>[2x]XETAAFAALRKPVDVAFGRNYVPTWAFDHIKYFNGGNEIQLHLDKYTGTGFQSKGSYLFGHFSMQMKLVPGDSAGTVTAFYLSSQNSEHDEIDFEFLGNRTGQPYIL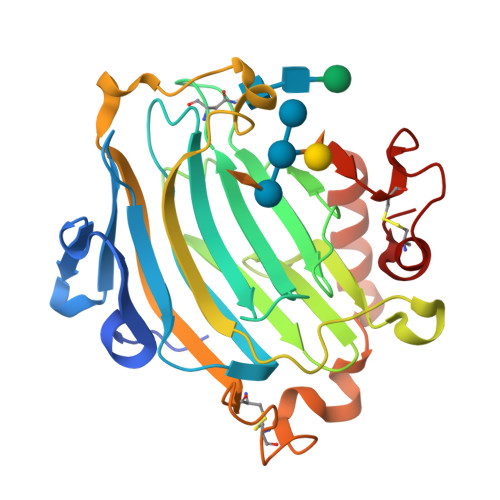QTNVFTGGKGDREQRIYLWFDPTKEFHYYSVLWNMYMIVFLVDDVPIRVFKNCKDLGVKFPFNQPMKIYSSLWNADDWATRGGLEKTDWSKAPFIASYRSFHIDGCEASVEAKFCATQGARWWDQKEFQDLDAFQYRRLSWVRQKYTIYNYCTDRSRYPSMPPECKRDRDI>[5x]MIVADSECRAELKDYLRFAPGGVGDSGPGEEQRESRARRGPRGPSAFIPVEEVLREGAESLEQHLGLEALMSSGRVDNLAVVMGLHPDYFTSFWRLHYLLLHTDGPLASSWRHYIAIMAAARHQCSYLVGSHMAEFLQTGGDPEWLLGLHRAPEKLRKLSEINKLLAHRPWLITKEHIQALLKTGEHTWSLAELIQALVLLTHCHSLSSFVFGCGILPEGDADGSPAPQAPTPPSEQSSP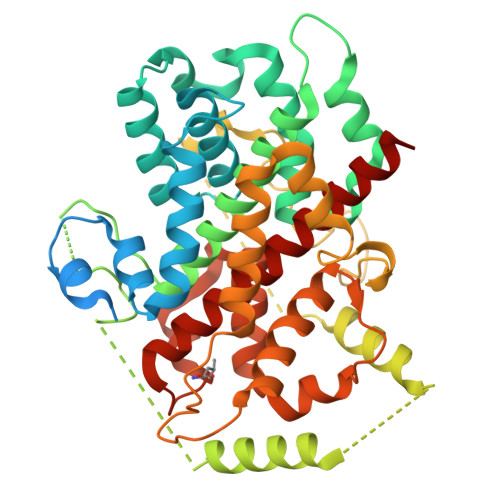PSRDPLNNSGGFESARDVEALMERMQQLQESLLRDEGTSQEEMESRFELEKSESLLVTPSADILEPSPHPDMLCFVEDPTFGYEDFTRRGAQAPPTFRAQDYTWEDHGYSLIQRLYPEGGQLLDEKFQAAYSLTYNTIAMHSGVDTSVLRRAIWNYIHCVFGIRYDDYDYGEVNQLLERNLKVYIKTVACYPEKTTRRMYNLFWRHFRHSEKVHVNLLLLEARMQAALLYALRAITRYMT>[2x]MLKIQAYFNETADLPCQFANSQNQSLSELVVFWQD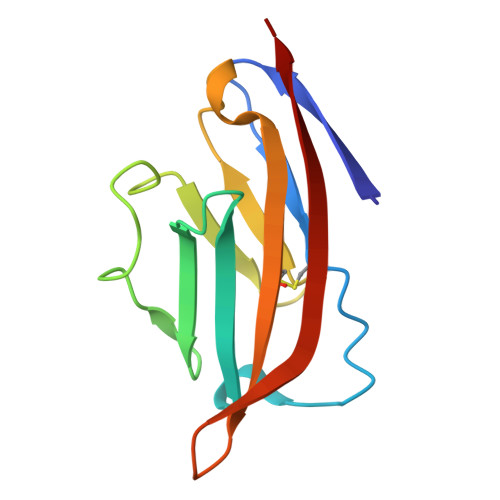QENLVLNEVYLGKEKFDSVHSKYMGRTSFDSDSWTLRLHNLQIKDKGLYQCIIHHKKPTGMIRIHQMNSELSVLA>GPLGSYGSRIEREQHHLIESIEKSTQYMAKRRIGALISVARDTGMDDYIETGIPLNAKISSQLLINIFIPNTPLHDGAVIIKGNEIASAASYLPLSD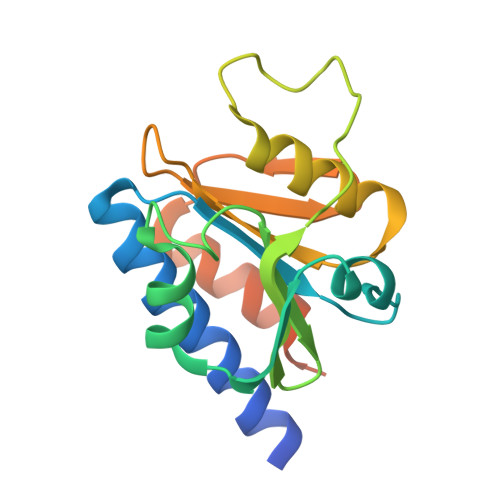SPFLSKELGTRHRAALGISEVTDSITIVVSEETGGISLTKGGELFRDVSEEELHKILLKELVTVTAKKPSIFSKWKGGKSE[2x]>[14x]GSSY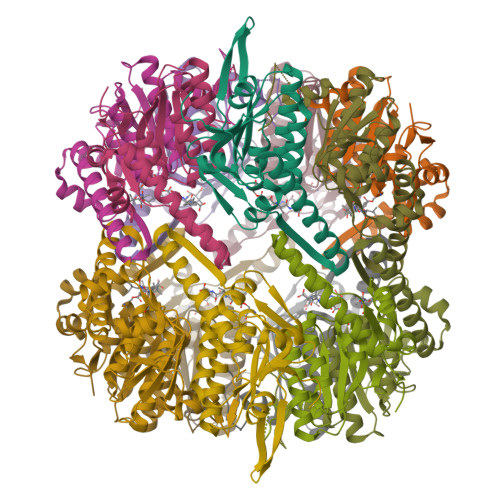SDKRDQYAPHMALVPMVVEQTTRGERSYDIYSRLLKERIIFLTGQVEDHMANLVAAQMLFLEAENPEKDIFLYINSPGGVITAGMSIYDTMQFIKPDVSTICMGQACSMGAFLLTAGAKGKRICLPNSRVMIHQPLGGFQGQATDIEIHAQEILKVKSRMNELMAKHTGRPIEEIAKDTERDRFLSADEAVEYGLVDKIFTHRD> SNAPRGCDILIVYSPDAEEWCQYLQTLFLSSRQVRSQKILTHRLGPEASFSAEDLSLFLSTRCVVVLLSAELVQHFHKPSLLPLLQRAFHPPHRVVRLLCGVRDSEEFLDFFPD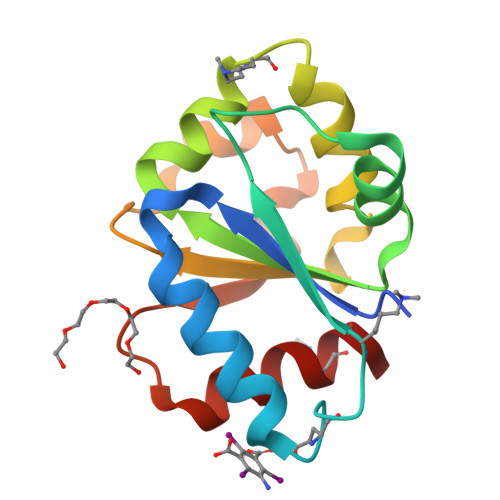WAHWQELTCDDEPETYVAAVKKAIS>[2x]LHLDQTPSRQPIPSEGLQLHLPQVL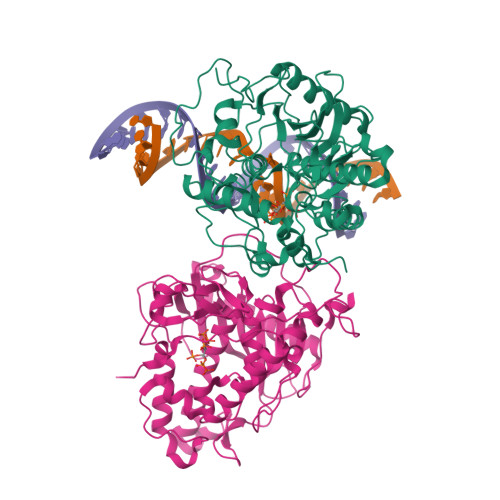ADAVSRLVLGKFGDLTDNFSSPHARRKVLAGVVMTTGTDVKDAKVISVSTGTKCINGEYMSDRGLALNDCHAEIISRRSLLRFLYTQLELYLNNKDDQKRSIFQKSERGGFRLKENVQFHLYISTSPCGDARIFSPHEPILEEPADRHPNRKARGQLRTKIESGQGTIPVRSNASIQTWDGVLQGERLLTMSCSDKIARWNVVGIQGSLLSIFVEPIYFSSIILGSLYHGDHLSRAMYQRISNIEDLPPLYTLNKPLLSGISNAEARQPGKAPNFSVNWTVGDSAIEVINATTGKDELGRASRLCKHALYCRWMRVHGKVPSHLLRSKITKPNVYHESKLAAKEYQAAKARLFTAFIKAGLGAWVEKPTEQDQFSLTP> MDGSGEQPRGGGPTSSEQIMKTGALLLQGFIQDRAGRMGGEAPELALDPVPQDASTKKLSESLKRIGDELDSNMELQRMIAAVDT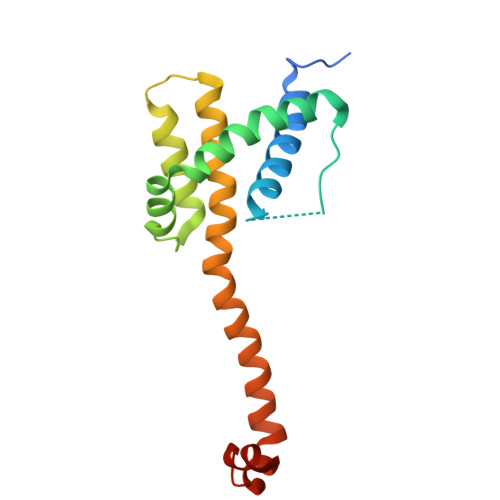DSPREVFFRVAADMFSDGNFNWGRVVALFYFASKLVLKALSTKVPELIRTIMGWTLDFLRERLLGWIQDQGGWDGLLSYGSS(2~{S},3~{S},4~{R},5~{R})-5-(6-aminopurin-9-yl)-3,4-bis(oxidanyl)-~{N}-piperidin-4-yl-oxolane-2-carboxamide | C15 H21 N7 O4 | 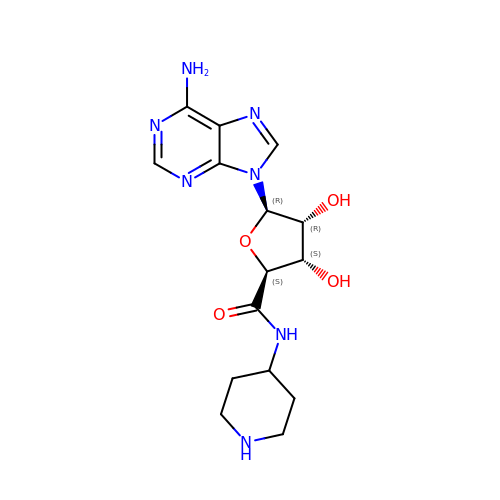MPKBIMHULNDLPU-BQVMBELUSA-N> YKDGDQCETSPCQNQGKCKDGLGEYTCTCLEGFEGKNCELFTRKLCSLDNGDCDQFCHEEQNSVVCSCARGYTLADNGKACIPTGPYPCGKQTLER;> IVGGQECKDGECPWQALLINEENEGFCGGTILSEFYILTAAHCLYQAKRFKVRVGDRNTEQEEGGEAVHEVEVVIKHNRFTKETYDFDIAVLRLKTPITFRMNVAPACLPERDWAESTLMTQKTGIVSGFGRTHEKGRQSTRLKMLEVPYVDRNSCKLSSSFIITQNMFCAGYDTKQEDACQGDSGGPHVTRFKDTYFVTGI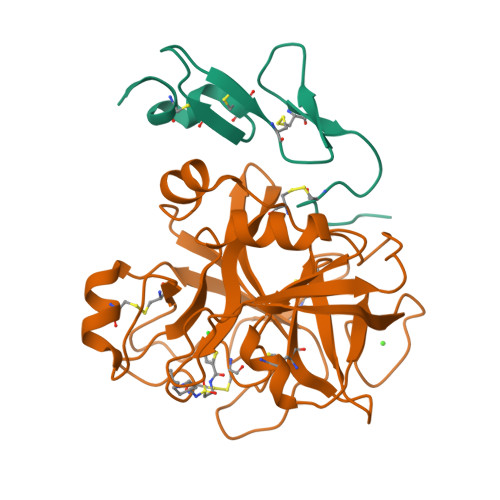VSWGEGCARKGKYGIYTKVTAFLKWIDRSMKTRGLPKAKSHAPEVITSSPLK>MVECSGNLFTQRTGTITSPDYPNPYPKSSECSYTIDLEEGFMVTLQFEDIFDIEDHPEVPCPYDYIKIKAGSKVWGPFCGEKSPEPISTQSHSIQILFRSD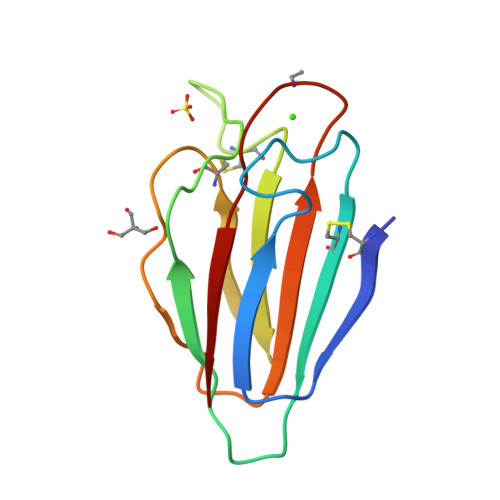NSGENRGWRLSYRA[2x]> MELKHSISDYTEAEFLQLVTTICNADTSSEEELVKLVTHFEEMTEHPSGSDLIYYPKEGDDDSPSGIVNTVKQW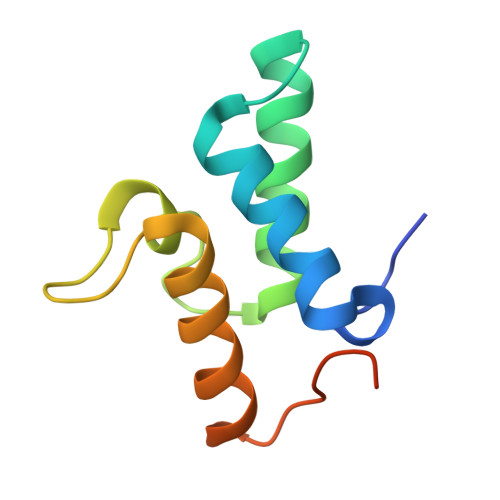RAANGKSGFKQGLEHHHHHH>[2x]GRTNLIVNYLPQNMTQDELRSLFSSIGEVESAKLIRDKVAGHSLGYGFVNYVTAKDAERAINTLNGLRLQSKTI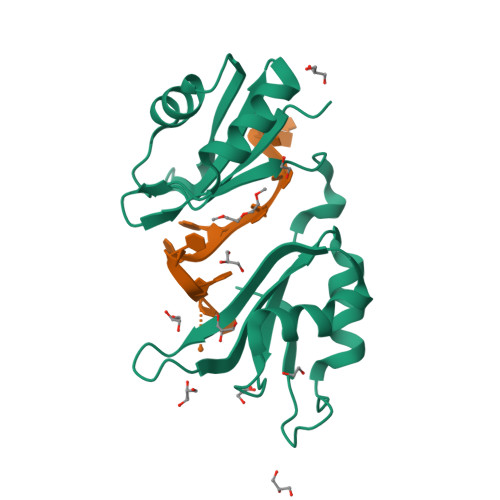KVSYARPSSEVIKDANLYISGLPRTMTQKDVEDMFSRFGRIINSRVLVDQTTGLSRGVAFIRFDKRSEAEEAITSFNGHKPPGSSEPITVKFAANLEHHHHHH> MGVGGDPAVALPHRRFEYKYSFKGPHLVQSDGTVPFWAHAGNAIPSSDQIRVAPSLKSQRGSVWTKTKAAFENWEVEVTFRVTGRGRIG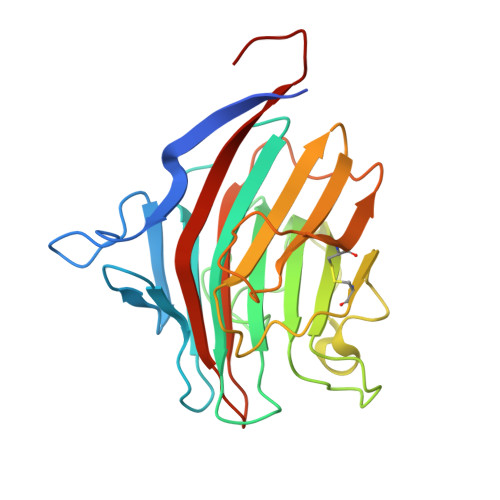ADGLAIWYAENQGLEGPVFGSADLWNGVGIFFDSFDNDGKKNNPAIVIIGNNGQIHYDHQNDGASQALASCQRDFRNKPYPVRAKITYYQNTLTVMINNGFTPDKNDYEFCAKVENMIIPAQGHFGISAATGGLADDHDVLSFLTFQLTEPGKEPPTP>[2x]MTNDYNTPLADTNLFKPI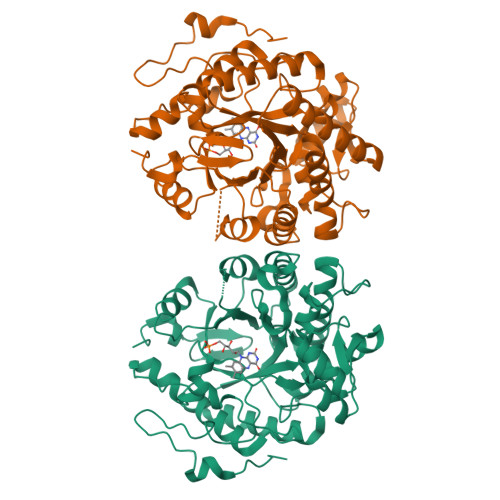KVGKIELKNRLVFPPTTRFRNTSDFVATDSMLSYYSQRAENNGGLLITEATFGAPQFGLYQNGPMIYTDRQVEAWKKIVEEVHKKGSHISMQLWNLGRAADPKLLKEHGLPFLAPSALYFSEESKKAAEEAGNEVQAMTLEQIEQTKKDYVNAAKNAIQKAGFDMVEVHSAHGYLLDQFIQTTANKRTDKYGGSIENRARLLLEVIDLVIEAVGADHVAVRLSPYATFQGSGGVDAEVHPIAQFGYILSELERRAKEGKRLAYVSIVEPRVNGIADAPENSEDNSWMLQIWKGVVLRSGGYLSEKGIAHLIKDVNADDRTLIGCSRYFTSNPDLPNRLRDGLPLTPYDRSRFYKIFSNDGYLTWGKYGEPEQPSDSAIALKTPQPLA Glucuronoyl esterases from carbohydrate esterase family 15 (CE15) have been proposed as an aid in reducing this recalcitrance by cleaving ester bonds found between lignin and glucuronoxylan. Only PvCE15 proved amenable to crystallization, and its structure was solved both as an apo protein and in complex with GlcA and GalA, respectively. PvCE15 has an α-/β-hydrolase fold like previously determined CE15 structures, consisting of a three-layer sandwich with a solvent-exposed cleft comprising the active site. The catalytic triad (Asp353-His406-Ser264) and oxyanion-stabilizing arginine (Arg265, oxyanion hole), whose positions and roles have been established in previous work on CE15 GEs, are conserved in PvCE15.

A complex structure with GalA was obtained by soaking with neutralized GalA, which revealed a binding pose distinct from the GlcA-binding pose, where the pyranose ring is flipped, resulting in the anomeric hydroxyl pointing into the cleft and positioned where the GlcA O4 is found. Distinctly, the carboxylate of the uronate is positioned out of the presumed catalytic center, with the C6 far from the catalytic serine (3.9 Å), but it is still positioned by the oxyanion-stabilizing arginine (Arg265) through one of its Nη atoms. A water molecule is found occupying the presumed catalytic center and is 3.2 Å away from the C6 of the uronate, which could suggest a water-mediated mechanism for this substrate. This orientation for GalA has also been observed with OtCE15A from Opitutus terrae, which has a similar preference for MeGlcA and MeGalA substrates, possibly suggesting a water-mediated mechanism for GalA substrates that is distinct from the mechanism utilized for GlcA substrates. However, the complexes obtained are only of the products of the reactions which may bind in a different orientation than required for catalysis. The complex structure of PvCE15 with GalA is found in a binding pose distinct from that of GlcA, where the carboxylate is positioned out of the catalytic center and could suggest a water-mediated mechanism for this substrate distinct from the serine adduct previously observed with OtCE15A and proposed for other CE15 members with GlcA substrates. The analogous pose was also observed in OtCE15A using a catalytically crippled variant, where the catalytic serine was replaced with alanine (S267A), and the difference in GalA versus GlcA positioning was speculated to be an artifact of residue substitution or the presence of DMSO solvent molecules present. However, this new observation of GalA also with the wild type PvCE15 reinforces the proposal of a distinct water-mediated mechanism for this substrate, especially for CE15 members with similar activity on GalA and GlcA esters. To investigate this, we obtained crystal structures of PvCE15 in complexes with both ligands.

>[2x]MGSSHHHHHHSSENLYFQGHSKSPRKDYAKLANYDESKVPQYTLPSVLMCHDGEMVQTKEQWEQKRRPEILNLFTTYMFGKAPVLKHKLPCTVSRINEKALNGRATRKEITIQLTDDPQGPHIDLQLYLPNHVSGKIPVFLGISFMPNYTIYDDPDLSVPEITDEKMKKRSFRGSMDKSWQLDKILEHGYGLATFCYNDVDPDFDDDFQNGVHPYYYEKGQNFPDPDQWGSIAAWAWGMSRAMDYLETDKKVDAKKVAVIGHSRLGKTAVWAGASDPRFALVISGNSGCCGVAISRRCFGETVEAMNVRFPHWFCGNYKQFNDREKYLPFDQHELVALIAPRPIYIASAEEDNWSDQKGEFLGGKGAEPVYALYGLGGIGCEEMPPVDTPYMNGPIAYHNRKGPHAVLPYDWEQFLRFADKYFKNK> GAMGKVTHSIHIEKSDTAADTYG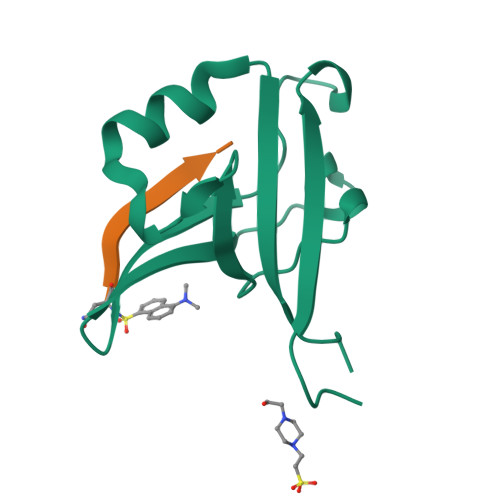FSLSSVEEDGIRRLYVNSVKETGLASKKGLKAGDEILEINNRAADALNSSMMEDFFSQPSVGLLVRTYPEL;> NKDKEYYV>MGLPPLLSLPSNSAPRSLGRVETPPEVVDFMVSLAEAPRGGRVLEPACAHGPFLRAFREAHGTAYRFVGVEIDPKALDLPPWAEGILADFLLWEPGEAFDLILGNPPYGIVGEASKYPIHVFKAVKDLYKKAFSTWKGKYNLYGAFLEKAVRLLKPGGVLVFVVPATWLVLEDFALLREFLAREGKTSVYYLGEVFPQKKVSAVVIRFQKSGKGLSLWDTQESESGFTPILWAEYPHWEGEIIRFETEETRKLEISGMPLGDLFHIRFAARSPEFKKHPAVRKEPGPGLVPVLTGRNLKPGWVDYEKNHSGLWMPKERAKELRDFYATPHLVVAHTKGTRVVAAWDERAYPWREEFHLLPKEGVRLDPSSLVQWLNSEAMQKHVRTLYRDFVPHLTLRMLERLPVRREYGFHTSPE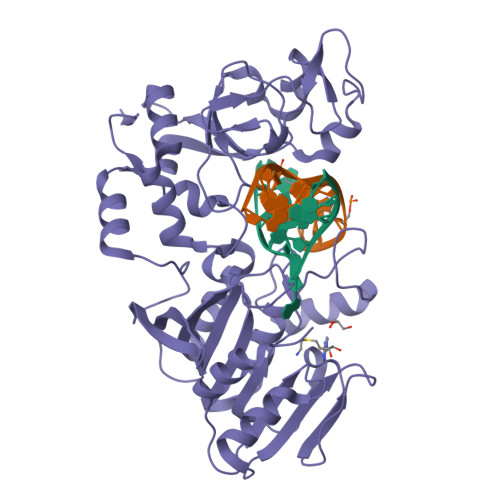SARNF[2x]>[4x]MKELIYIEEPKILFAHGQKCTDARDGLALFGPLNNLYGIKSGVIGTKQGLKIFRDYLDHIQKPIYNSNSITRPMFPGFEAVFDCKWESTGITFKEVTNEDIGKFLY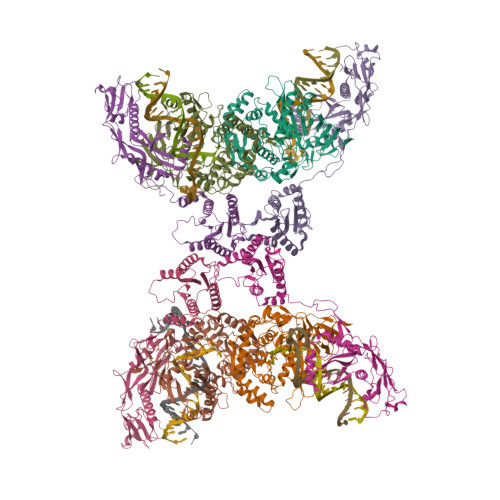NSSTHKRTYDLVSLFIDKIISANKNEDENVDVWFVIVPDEIYKYCRPNSVLPKEMVQTKALMSKSKAKSFRYEPSLFPDINIELKEQEKEAETYNYDAQFHDQFKARLLKHTIPTQIFRESTLAWRDFKNAFGLPIRDFSKIEGHLAWTISTAAFYKAGGKPWKLSDVRNGVCYLGLVYKKVEKSKNPRNACCAAQMFLDNGDGTVFKGEVGPWYNPKNGQYHLEPKEAKALLSQSLQSYKEQIGEYPKEVFIHAKTRFNHQEWDAFLEVTPKETNLVGVTISKTKPLKLYKTEGDYTILRGNAYVVNERSAFLWTVGYVPKIQTALSMEVPNPLFIEINKGEADIKQVLKDILSLTKLNYNACIFADGEPVTLRFADKIGEILTASTDIKTPPLAFKYY;>[4x]MRNKIFISHATPDDNDFTRWLALKLIGLGYEVWCDILFLDKGVDFWSNIEKVIREDTCKFLLVSSSYSNQREGVLKELAVAAKVKKQLKDDKFIIPLAIDEQLSYDDINIDIVRLNAIDFKMSWARGLKDILEAFEKQKVPKEVADASKSNLLYQQIFLHDKSVIEKEEIYDSNWLSILSFPEELRFHEYNWMLPKRFDVRELTFPAVRYKNYLCTFAWAYDFTYHLPKTETYHKSKTIRIPTEEILSGSYDSNFIRNAECKRLIVQLLNKAFELRMKDKEVQEYEMSNKTAYWLEKGKLEKDKFEKTMLVGKQKDKNWHFAISGASKLYPFPVLMISSHIFFTADGKKLIDSSSVQHSSRRRQGKNWWNNTWRTKLLAFIKYLSDDDTSFYLEMGSEEKVFVSNEPVKFKGNVSYNI> ASTFSGVQSLPKFEIHDVRDDPAEGTMTRVAVDGKLLLISQYPQLGPRKVDPNDLSPQFDADRRISVRLRHVDLAY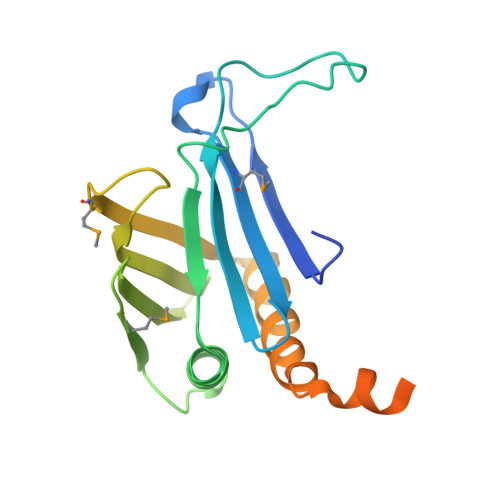LVGVCKERVPRHRMETKAYTLDFEKSAQGYHLHGKVHRVASQRMEDWSVKFDNHFAVTLEHFLESALDESFGFRQHYATRAAEGGEKIAATSSAEGGARRKRSVSDTSRYH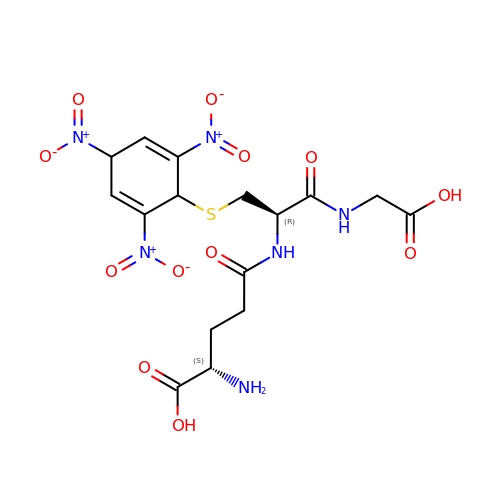1-(S-GLUTATHIONYL)-2,4,6-TRINITROCYCLOHEXA-2,5-DIENE | C16 H20 N6 O12 S | VQUXYLXGOSJDJJ-OSGJSWLFSA-N>[2x]AESLPDLKIEKLDEGVYVHTSFEEVNGWGVVPKHGLVVLVNAEAYLIDTPFTAKDTEKLVTWFVERGYKIKGSISSHFHSDSTGGIEWLNSRSIPTYASELTNELLKKDGKVQATNSFSGVNYWLVKNKIEVFYPGPGHTPDNVVVWLPERKILFGGCFIKPYGLGNLGDANIEAWPKSAKLLKSKYGKAKLVVPSHSEVGDASLLKLTLEQAVKGLNESKKPSKPSN

β-Lactam-containing compounds remain the most important antibiotics in clinical use, but their effectiveness is threatened by increasing resistance. β-Lactam resistance is most importantly mediated by serine- and zinc-dependent metallo-β-lactamases (SBLs and MBLs, respectively), which catalyze β-lactam hydrolysis. B1 MBLs (e.g., imipenemase [IMP], Verona integron-encoded MBL [VIM], and New Delhi MBL [NDM] types) are the most clinically relevant MBLs; these MBLs catalyze hydrolysis of almost all β-lactams, including the latest generations of cephalosporins and carbapenems. Crystal structures reveal that MBLs have a characteristic αβ/βα sandwich fold, that they possess conserved zinc ion binding sites, and that loops flanking the active site are involved in ligand binding. We report systematic studies on the inhibition of four clinically relevant MBLs (IMP-1, VIM-2, SPM-1, and NDM-1) and the model MBL BcII by the four captopril stereoisomers and both enantiomers of a captopril derivative, 1-(2-mercaptobenzoyl)pyrrolidine-2-carboxylic acid (d- and l-MBP).

We determined high-resolution crystal structures for d- and l-captopril in complex with IMP-1 (1.71- and 2.01-Å resolutions, respectively), VIM-2 (1.40- and 1.20-Å resolutions, respectively), and BcII (1.18- and 1.10-Å resolutions, respectively). For the IMP-1–d-captopril and IMP-1–l-captopril structures, the ligands were modeled and refined with 100% occupancy in chain A, but the residual density present in chain B was interpreted as too weak (<50% occupancy) to include in the model. In all cases, cysteine oxidation during crystallization could be prevented by the addition of tris(2-carboxyethyl)phosphine (TCEP) (except for IMP-1, for which cysteine oxidation in the absence of TCEP was not observed). As observed for our MBL–d-captopril structures, the IMP-1–l-captopril structure has the inhibitor carboxylate positioned to form an electrostatic interaction with a conserved basic residue, i.e., Lys224. In all MBL–l-captopril structures (including those with IMP-1), the carboxylate is positioned to interact with the conserved asparagine (Asn233) from the L10 loop. IMP-1 is thus apparently a special case, i.e., both the l- and d-captopril isomers bind in similar modes with the inhibitor carboxylate positioned to interact with Lys224IMP-1. Second, the observation of a decreased number of hydrogen bonding/electrostatic interactions for l- over d-captopril generally reflects weaker inhibition. l-Captopril was observed to be more potent against IMP-1 than against the other MBLs tested, and its IC50 was only 3-fold higher than that of d-captopril. This observation of relatively potent inhibition of IMP-1 by l-captopril correlates with the observation that for IMP-1, but none of the other MBLs, the l-captopril carboxylate favors binding to Lys224IMP-1.>[3x]GPGSMTDAPGALAERRGNVMVITINRPEARNAVNAAVSIGVGDALEEAQHDPEVRAVVLTGAGDKSFCAGADLKAI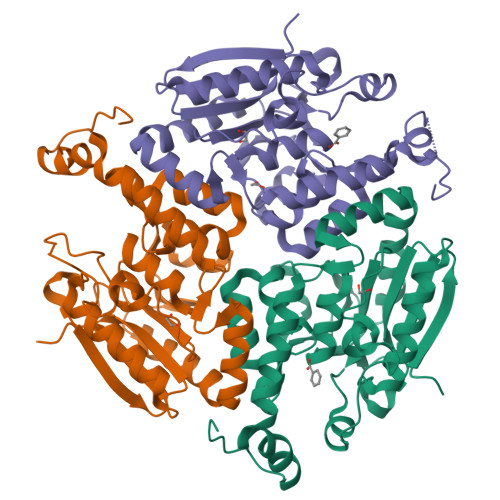ARRENLYHPDHPEWGFAGYVRHFIDKPTIAAVNGTALGGGTELALASDLVVADERAQFGLPEVKRGLIAAAGGVFRIAEQLPRKVAMRLLLTGEPLSAAAARDWGLINEVVEAGSVLDAALALASAITVNAPLSVQASKRIAYGVDDGVVVGDEPGWDRTMREMRALLKSEDAKEGPRAFAEKREPVWQAR>QRCGEQGSNMECPNNLCCSQYGYCGMGGDYCGKGCQNGACWTSKRCGSQAGGATCTNNQCCSQYGYCGFGAEYCGAGCQGGPCRADIKCGSQAGGKLCPNNLCCSQWGFCGLGSEFCGGGCQSGACSTDKPCGKDAGGRVCTNNYCCSKWGSCGIGPGYCGAGCQSGGCD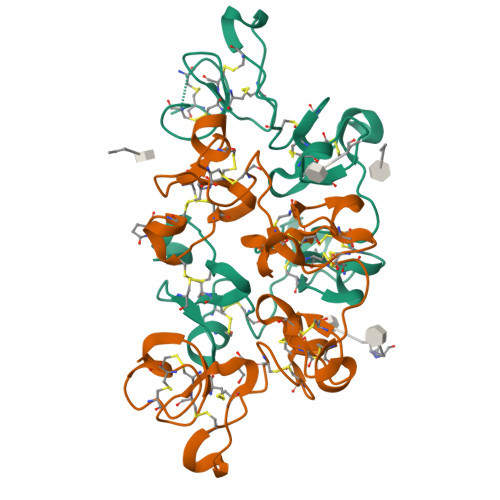G[4x]GLYCYL-L-ALPHA-AMINO-EPSILON-PIMELYL-D-ALANYL-D-ALANINE 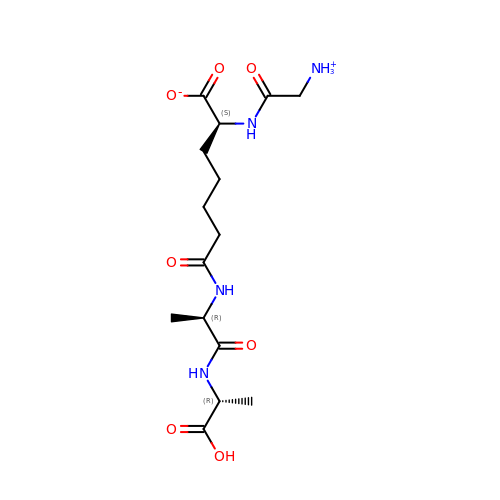| C15 H26 N4 O7 | RALBRZJHHGWNNU-BBBLOLIVSA-N>[2x]MISLADLQRRIETGELSPNAAIAQSHAAIEAREKEVHAFVRHDKSARAQASGPLRGIAVGIKDIIDTANMPTEMGSEI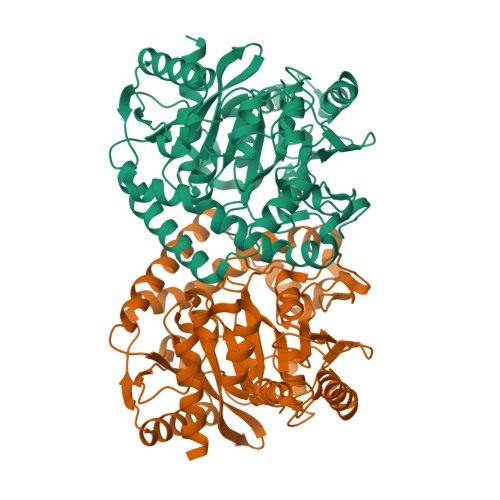YRGWQPRSDAPVVMMLKRAGATIIGKTTTTAFASRDPTATLNPHNTGHSPGASSSGSAAAVGAGMIPLALGTQTGGSVIRPAAYCGTAAIKPSFRMLPTVGVKCYSWALDTVGLFGARAEDLARGLLAMTGRSEFSGIVPAKAPRIGVVRQEFAGAVEPAAEQGLQAAIKAAERAGASVQAIDLPEAVHEAWRIHPIIQDFEAHRALAWEFSEHHDEIAPMLRASLDATVGLTPKEYDEARRIGRRGRRELGEVFEGVDVLLTYSAPGTAPAKALASTGDPRYNRLWTLMGNPCVNVPVLKVGGLPIGVQVIARFGNDAHALATAWFLEDALAKSG>MGIPKFFHFISERWPQISQLIDGSQIPEFDNLYLDMNSILHNCTHGDGSEVNSRLSEEEVYSKIFSYIDHLFHTIKPKQTFYMAIDGVAPRAKMNQQRARRFRTAMDAEKALQKAIENGDELPKGEPFDSNAITPGTEFMAKLTENLKYFIHDKITNDTRWQNVKVIFSGHEVPGEGQHKIMDYIRAIRAQEDYNPNTRHCIYGLDADLIILGLSTHDHHFCLLREEVTFGKRSSSVKTLETQNFFLLHLSILREYLALEFEEITDSVQFEYDFERVLDDFIFVLFTIGNDFLPNLPDLHLKKGAFPVLLQTFKEALQHMDGYINEQGKINLARFSIWLKYLSDFEYLNFEKKDIDVEWFNQQLENISLEGERKRTRMGKKLLMKQQKKLIGAVKPWLLKTVQRKVTSELQDADFEIFPLEDKELVRANLDFLKEFAFDLGLILAHSKSKDLYYFKLDLDSINXXXXXXXXXXXXXXXXXXXIYSERFVEWKDQYYKDKLDFSINDTDSLKEMTENYVGGLQWVLYYYYRGCPSWSWYYRYHYAPRISDVIKGIDQNIEFHKGQPFKPFQQLMAVLPERSKNLIPVVYRPLMYDEHSPILDFYPNEVELDLNGKTADWEAVVKISFVDQKRLVEAMAPYDAKLSPDEKKRNSFGTDLIFIFNPQVDTVYKTPLAGLFNDIEHNHCIEREFIPESMENVKFLFGLPKGAKLGASSLAGFPSLKTLPLTAELAYNSSVVFNFPSKQQSMVLHIQDLYKENGISLSDLAKRHMGKIVYSRWPFLRESKLLSLITEETVYEGVKSGKLTKVIERKPQDFERKEFRELKMTLKSNYQRTKAILLDDISALAKVVPVNGLVRNSDGSYSKSFNETIEYYPLQLIVEDVKNKDERYIEKEPLPINKEFPKGSKVVFLGDYAYGGEATVDGYNSETRLKLTVKKGSLRAEPNIGKVRAKLDSQALRFYPTQVXXXXXXXXXXXXXXXXXXXSSAEADSILKTVADWLSEARKPFVVVSLESDSLTKASMAAVESEIIKYVSLPDSSEQKKLAKVPREAILNAESSYVLLRSQRFHLGDRVMYIQDSGKVPLHSKGTVVGYTSIGKNVSIQVLFDNEIIAGNNFGGRLQTRRGLGLDSSFLLNLSDRQLVYHSKA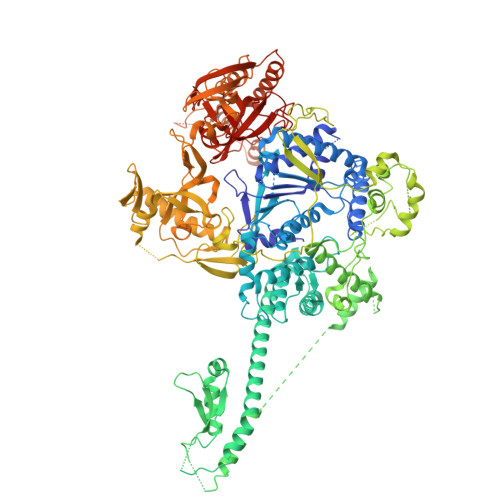SLEHHHHHH[4x]>RSSPNKGLHILDRSEWLGEPPSGKYPHLKLPVSNIIIHHTATEGCEQEDVCIYRMKTIQAFHMKSFGWVDIGYNFLVGGDGQIYVGRGWHIQGQHVNGYGAISVSIAFIGTFVNMEPPARQIEAAKRLMDEGVRLHRLQPDYHIYAHRQLSPTESPGQKLFELMQNWPRFTQDPTSLES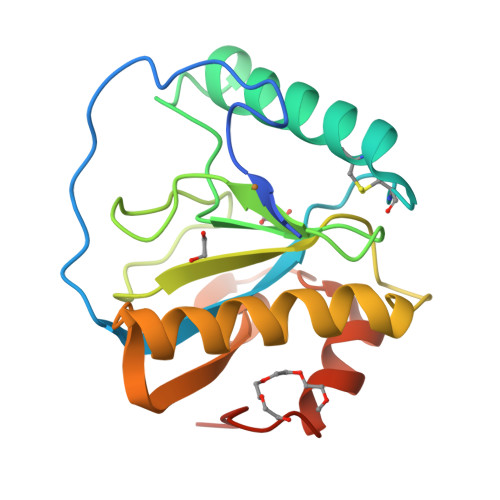R[2x]3-OXO-3-[(3-OXOPROPYL)SULFANYL]PROPANE-1-THIOLATE 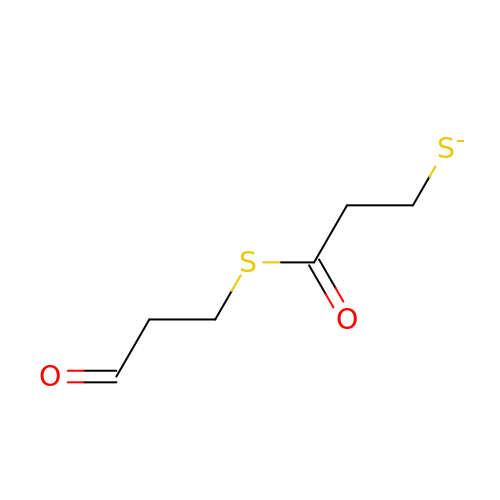| C6 H9 O2 S2 | LHLHVBHXBHTTIV-UHFFFAOYSA-M>MQRARPGELVEVIMFRPTGKARVSNLDESMAMEFTDLRTRAMSSAAMIRQSVAAKTLLIENEDGKGSTRMEVQDFMKRFHMHASEDDKTGSPSTAWGTLRFPTKEATAPYLRLSVNDDPEDALLFVKAMLAQKYGETYDRPSLILSVTGGARNFTLPPRLETAIAKGLRLAAQRTNAWVVTGGTNTGVMKLTGQIMEALSKTQSHFIPPTIGIATYGVIIGGDDMTRGEPPKIGLEYEMHKKDPPKTTPLDDNHNLFLLVDDGSTNKFGKEIKFRAAFENAAGQAFAAPVVTIVVQGGPGTLGTALQAVRQGTPIVVVDGSGLAADVLAYAYNFMHNPLTRFKSYTIDDLRQKVAQTFNPKSSQQLTNLLDSALECVQDPNLVVVYSLQESGIDEFDDCILKAIFSSQGKLGNKLKQAMYFDQLDVAKRALSEASKNGQHNEIAACINDNLMAAMMHNKPHFVELYLGFDAKIYELKPSEEVAKTNITALDELPSFALAIEELYKREAKKPHSHVQRLVSLSNTDVLGRHYRVSTQRGDGTTRRIGRDLANTRAYNVLRMDQIFARLVSKDFSVNRDFTIYDSKYDKVPGIQFRRTAQASHMLFLWAICLDRFRMARHFWLIGDQSIINALVASRILERLSTHRALQGPHLAEERAKMQHNAKKFEELAVGVLGECHGSDSHMASEMLHSKNDMFNKKNAINIAYDAKSLAFLSHPATQSVINADWYGHLKSVTSFWAVLFAFFFPFFVLPFINFSEDHAEQQVEAPRDFFTDAPRSSHSANSTTSGAHRLRRKFAKFYSAPYTRFISDLLSHFVLCVVTSYFVLDKLEDTISAIEWILLVWFVALLLEELRQMIFCDGIAEYISDTWNRLDLIMITLFFVGFFTHASDPSNQDSKVVSKGIHAFLVVVLWLRFMRYYALSKNLGPKLIMMMEMMKDVSTFVFLLLIFLIGYGVAAQSLLSPDEDFSSRTFIGVLFRPYFQIYGELFLDDLNSEANCLGDTPFTECSRETVRMVPFFLAVYILGSNVLLVNLLIAMFNDTYMKVQEAAEDLWRKQNYELCAEYKDRPFLPAPFILLAHVHMLFMRLLRLCGVHTQEHEKIQDDETKRKITTFEALNTDKFLRRWERERQEMLEARVKMTNDNVVQAMGMMDQLLEHMISFRFSLDQQATKIKQEIRDDGLPSTEPTGLVSRTPSQPINRLNSAVAVHGHTAEAAEWYVPPEEYPKSGGVKRYLIDASMVPLSIMCPSYDPVEYTHPSVAAQPVWADPADPRKIKFNVKDEVNGKVVDRTSCHPSGISIDSNTGRPINPWGRTGMTGRGLLGKWGVNQAADTVVTRWKRSPDGSILERDGKKVLEFVAIQRQDNKMWAIPGGFVDNGEDVALTSGREFMEEALGMGTSADLMSAESKDSLAALFSSGTIVARIYCEDPRNTDNAWVETTCVNFHDESGRHAARLKLQGGDDAEHARWMMVHGGLNLFASHRTLLQHVTSALNAYF[4x]

We investigated a TRPM2 chanzyme from choanoflagellates that integrates two seemingly incompatible functions into a single peptide: a channel module activated by ADP-ribose with high open probability and an enzyme module (NUDT9-H domain) consuming ADP-ribose at a remarkably slow rate. Using time-resolved cryogenic-electron microscopy, we captured a complete series of structural snapshots of gating and catalytic cycles, revealing the coupling mechanism between channel gating and enzymatic activity. The slow kinetics of the NUDT9-H enzyme module confers a self-regulatory mechanism: ADPR binding triggers NUDT9-H tetramerization, promoting channel opening, while subsequent hydrolysis reduces local ADPR, inducing channel closure. The structures of srTRPM2 exhibit a characteristic TRPM architecture, from top to bottom, a transmembrane domain (TMD) layer containing the ion-conducting pore, a signal transduction layer consisting of MHR3/4 domain and the C-terminal rib helix, and an ADPR-sensing layer consisting of the N-terminal MHR1/2 domain and the C-terminal NUDT9-H domain.

A cation binding site is found between the MHR3/4 domain and the Rib helix of each subunit, termed MgMHR. This site does not distinguish between Ca2+ or Mg2+ either and is unique to srTRPM2 as the key residue, E1114, is not conserved. Replacing E1114 with alanine eliminated cation binding at MgMHR, resulting in a reduced rotational movement of the intracellular domain around the symmetry axis when ligands were bound, as compared to the wild-type (WT) protein. The E1114A mutation had no obvious effect on macroscopic currents. However, single-channel analysis showed a small decrease in channel open probability and a small increase in channel close rate, revealing a regulatory role of this cation binding site on channel gating.> GPGSEFRPQPLPPGWERRVDDRRRVYYVDHNTRTTTWQRPTMESVRNFEQWQSQRNQLQGAMQQFNQRYLYSASMLAAENDPYGPLPPGWEKRVDSTDRVYFVNHNTKTTQWEDPRTQGLQNEEPLPEGWEIRYTREGVRYFVDHNTRTTTFKDPRNGKSSVTKGGPQIAYERGFRWKLAHFRYLCQSNALPSHVKINVSRQTLFEDSFQQIMALKPYDLRRRLYVIFRGEEGLDYGGLAREWFFLLSHEVLNPMYCLFEYAGKNNYCLQINPASTINPDHLSYFCFIGRFIAMALFHGKFIDTGFSLPFYKRMLSKKLTIKDLESIDTEFYNSLIWIRDNNIEECGLEMYFSVDMEILGKVTSHDLKLGGSNILVTEENKDEYIGLMTEWRFSRGVQEQTKAFLDGFNEVVPLQWLQYFDEKELEVMLCGMQEVD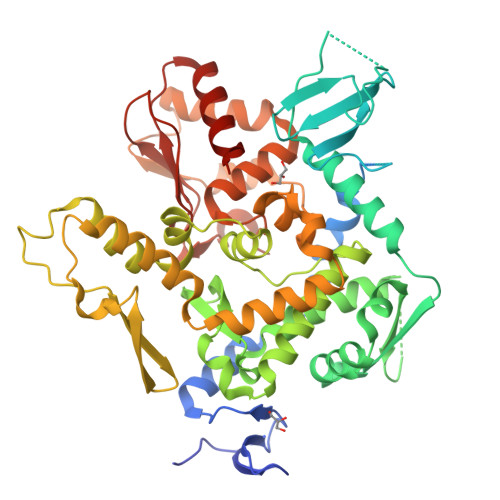LADWQRNTVYRHYTRNSKQIIWFWQFVKETDNEVRMRLLQFVTGTCRLPLGGFAELMGSNGPQKFCIEKVGKDTWLPRSHTCFNRLDLPPYKSYEQLKEKLLFAIEETEGFGQE> SMFLPPPECPVFEPSWEEFADPFAFIHKIRPIAEQTGICKVRPPPDWQPPFACDVDKLHFTPRIQRLNELEAQTRVKLGGGGASDYTLRTFGEMADAFKSDYFNMPVHMVPTELVEKEFWRLVSTIEEDVTVEYGADIASKEFGSGFPVRDGKIKLSPEEEEYLDSGWNLNNMPVMEQSVLAHITADICGMKLPWLYV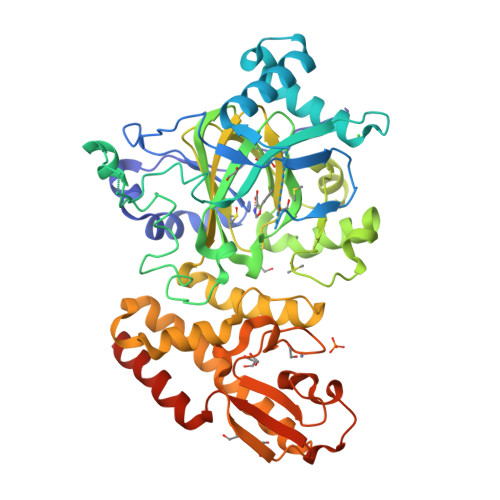GMCFSSFCWHIEDHWSYSINYLHWGEPKTWYGVPGYAAEQLENVMKKLAPELFVSQPDLLHQLVTIMNPNTLMTHEVPVYRTNQCAGEFVITFPRAYHSGFNQGFNFAEAVNFCTVDWLPLGRQCVEHYRLLHRYCVFSHDEMICKMASKADVLDVVVASTVQKDMAIMIEDEKALRETVRKLGVIDSERMDFELLPDDERQCVKCKTTCFMSAISCSCKPGLLVCLHHVKELCSCPPYKYKLRYRYTLDDLYPMMNALKLRAESYNEWALNVNEALEAKI>MLGLKTSIIGRRVIYFQEITSTNEFAKTSYLEEGTVIVADKQTMGHGALNRKWESPEGGLWLSIVLSPKVPQKDLPKIVFLGAVGVVETLKEFSIDGRIKWPNDVLVNYKKIAGVLVEGKGDKIVLGIGLNVNNKVPNGATSMKLELGSEVPLLSVFRSLITNLDRLYLNFLKNPMDILNLVRDNMILGVRVKILGDGSFEGIAEDIDDFGRLIIRLDSGEVKKVIYGDVSLRFL[2x];>MVVSENVVSAPMPGKVLRVLVRVGDRVRVGQGLLVLEAMKMENEIPSPRDGVVKRILVKEGEAVDT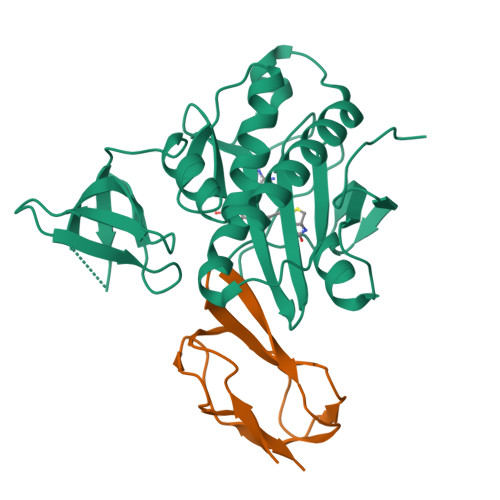GQPLIELG[2x]>[2x]EDFVDPWTVQTSSAKGIDYDKLIVRFGSSKIDKELINRIERATGQRPHHFLRRGIFFSHRDMNQVLDAYENKKPFYLYTGRGPSSEAMHVGHLIPFIFTKWLQDVFNVPLVIQMTDDEKYLWKDLTLDQAYSYAVENAKDIIACGFDINKTFIFSDLDYMGMSSGFYKNVVKIQKHVTFNQVKG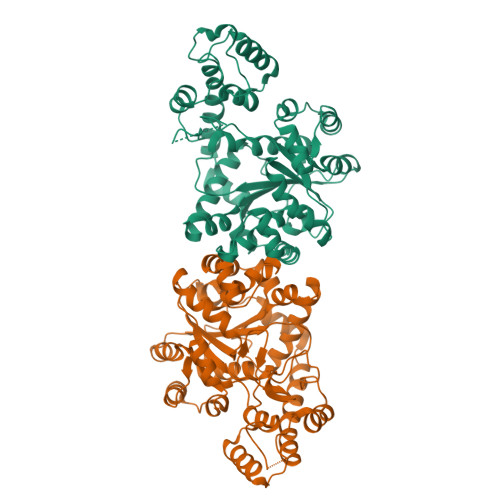IFGFTDSDCIGKISFPAIQAAPSFSNSFPQIFRDRTDIQCLIPCAIDQDPYFRMTRDVAPRIGYPKPALLHSTFFPALQGAQTKMSASDPNSSIFLTDTAKQIKTKVNKHAFSGGRDTIEEHRQFGGNCDVDVSFMYLTFFLEDDDKLEQIRKDYTSGAMLTGELKKALIEVLQPLIAEHQARRKEVTDEIVKEFMTPRKLSFDFQ Dye-decolorizing peroxidases (DyPs) are heme proteins with distinct structural properties and substrate specificities compared to classical peroxidases. Here, we demonstrate that DyP from the extremely radiation-resistant bacterium Deinococcus radiodurans is, like some other homologues, inactive at physiological pH. Structurally, DyP-type peroxidases also differ from the classical peroxidases. In contrast with the α-helix rich structures of the latter, DyPs are organized in two domains with a ferredoxin-like fold of four anti-parallel β-sheets surrounded by α-helices. A sequence analysis of DrDyP compared to four characterized and structurally determined members of the class V peroxidase family of DyPs, demonstrates that the proximal His heme ligand, and the four residues that are proposed to form the hydrogen peroxide binding pocket within this family of DyPs are conserved in DrDyP (H324, D189, R348, L373 and F375).

To gain more insight into the function of DyP from D. radiodurans, both DrDyP and DrDyPM190G were crystallized and structurally determined to 2.20 and 1.53 Å resolution, respectively. DrDyP possesses one and DrDyPM190G possesses two molecules in the asymmetric unit, respectively. The final model of DrDyP (residue 19–460) contains one heme molecule, two glycerols, three Magnesium ions and 45 waters. In total, DrDyP contain 12 α-helices and 10 β-strands, with the β-sheets located mainly in the interior of the protein and the α-helices on the surface of the protein. A superimposition of the two structures demonstrates that they are almost identical with an RMSD value of 0.28. The assumed catalytic residue in both structures (Asp189 and Arg248) and the axial His324 are well-aligned relative to the heme. Interestingly, we could observe one hydroxyl group and one water molecule within the hydrogen bonding distance to the iron and the catalytic Asp189 and Arg248 on the distal side of the heme for DrDyPM190. This was not observed for the DrDyP structure and can most likely be explained with the lower resolution of this structure. DrDyP is inactive at physiological pH, due to the fact that the heme adopts 6cLS state at pH 7.5, as shown using the resonance Raman experiments. Like BsDyP, DrDyP’s reduction potential is in the moderately high range, which along with the high amount of the catalytically inactive 6cLS heme iron may explain its poor performance as a peroxidase.

> KIDLDLDDIQATVLRERPEPYYGTHAMVRFDTAEGGRELLKRLLPHIASAEKWWDVKYAWTAAAISYEGLKKLGVPQDSLDSFPESFKVGMAGRAEHLFDVGENDPKHWEKPFGTGQVHLALTIFAENEENWQKALVIAEHELEATKGVTLLMREDFGAQPDSRNSLGYKDMISNPAIEGSGIKPFPGQGPAIKPGEFVLGYPGEAGVPLGMPKPEVLGKNGTFVALRKYHTNAGSFNRYLKENAEYTGGDAELLAAKLVGRWRSGAPLTLAPKEDDPELGHDPNRNNDFTYKNDPEGLEVPLGSHIRRMNPRDTKLELLTDVNIHRIIRRATAYGPAYDPKADSLAEDKVERGLYFIFISAKAMDTTEFLQKEWINKANFIGQGSERDPIVGLQDEDLTFTLPKEPVRQRLRGMDTFNVLRGGEYLFMPSLSALKWLSELK>GIDPFTMTPSEDFVVTDRGGIVENSHRVHAAVVDAKGRLLYALGNPTRMTLARSAAKPAQALAILETEGVAGYGFDDADIALMCASHSSEDRHIARTRAMLSKIKAEEADLRCGGHPSLSEMVNRSWIKQDFIPTAVCSNCSGKHVGMLAGARAIGAGTDGYHLPDHPMQGRVKRTVAELCDLDAGDVEWGTDGCNLPTPAFPLDRLGRIYAKLASAADGSDAGEGQSTRCAALAHIFRAMARHPEMVAGEGRYCTMLM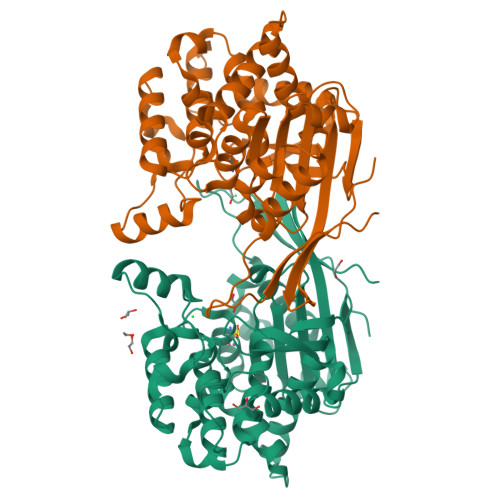RAFDGALVGKLGADASYAIGVRASDATRQLGTDGALGISVKIEDGNLEMLYAVVTELLERLGIGSPDVRSQLASFHHPQRVNTMGVTTGGVSFPFKLRGSKSNVDDPRLAAVAR[4x]> GGACGGCCGG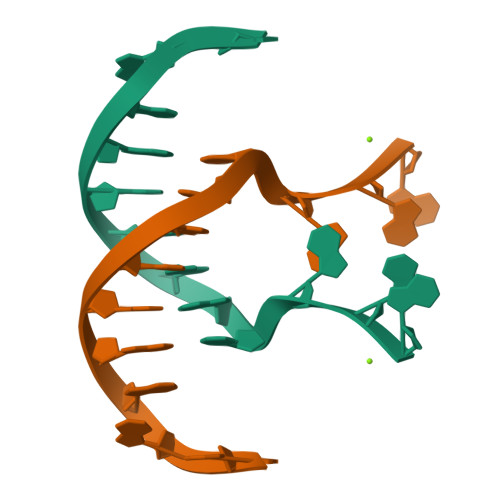GAG Here, we show that the protein FCHSD2 is a major activator of actin polymerization during CME. FCHSD2 is recruited to endocytic pits by the scaffold protein intersectin via an unusual SH3-SH3 interaction. When bound to the membrane, FCHSD2 activates actin polymerization by a mechanism that combines oligomerization and recruitment of N-WASP to PI(4,5)P2, thus promoting pit maturation.

The fourth SH3 domain of ITSN1 (SH3d) could pull down FCHSD2 SH3-2. Isothermal titration calorimetry (ITC) revealed a 248 nM (±75 nM) affinity (Kd) with a ∼1:1 stoichiometry. SH3 domains generally bind short proline-rich sequences rather than mediate domain-domain interactions. To understand how this unusual SH3-SH3 interaction occurs, we solved the crystal structure of the FCHSD2 SH3-2/ITSN1 SH3d complex at 3.4 Å. The structure revealed tandem binding between the SH3 domains with the canonical proline-binding interface of FCHSD2 SH3-2 interacting with the surface opposite to the proline-binding interface of ITSN1 SH3d. The domains form an extensive contact surface composed largely of hydrophobic residues and a few charge interactions. Double mutants on FCHSD2 SH3-2 (Y576S+F607S or V622K+L623K) were required to abolish the interaction to ITSN1 SH3d. On the other hand, single residue mutations on ITSN1 SH3d (I1078S, I1078K, R1119A, or R1119E) could abolish the interaction with FCHSD2 SH3-2. Additionally, mutation of residues located on crystal contacts (FCHSD2 SH3-2 N613 and D583; ITSN1 SH3d T1086) did not show any effect on binding. In agreement with the interface from the crystal structure, wild-type ITSN1 SH3d could efficiently recruit FCHSD2 to the mitochondria while the interface mutant ITSN1 SH3d R1119E could not.

>[4x]ASVCFVKALYDYEGQTDDELSFPEGAIIRILNKENQDDDGFWEGEFNGRIGVFPSVLVEELSA;>[4x]KKPEIAQVIASYTATGPEQLTLAPGQLILIRKKNPGGWWEGELQARGKKRQIGWFPANYVKLLSP>[2x]MKVRIATYASHSALQILKGAKDEGFETIAFGSSKVKPLYTKYFPVADYFIEEKYPEEELLNLNAVVVPTGSFVAHLGIELVENMKVPYFGNKRVLRWESDRNLERKWLKKAGIRVPEVYEDPDDIEKPVIVKPHGAKGGKGYFLAKDPEDFWRKAEKFLGIKRKEDLKNIQIQEYVL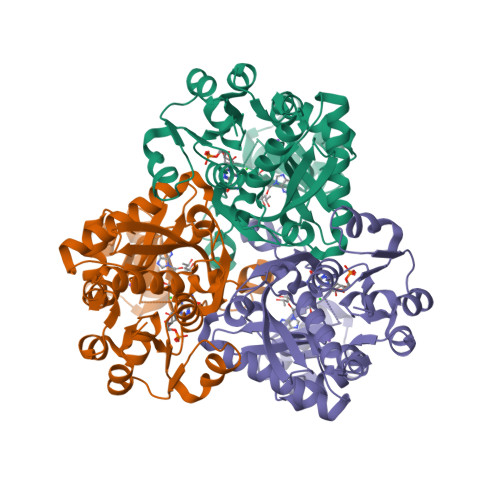GVPVYPHYFYSKVREELELMSIDRRYESNVDAIGRIPAKDQLEFDMDITYTVIGNIPIVLRESLLMDVIEAGERVVKAAEELMGGLWGPFCLEGVFTPDLEFVVFEISARIVAGTNIFVNGSPYTWLRYDRPVSTGRRIAMEIREAIENDMLEKVLT The surfaces of most bacteria and archaea are covered with a proteinaceous coat, the surface or S-layer, which is formed through the self-assembly of individual protein subunits into a regularly spaced, two-dimensional array. In C. difficile, the S-layer largely consists of a major S-layer protein, SlpA, which assembles into a paracrystalline array enveloping the cell. The major protein of the C. difficile S-layer, SlpA, is post-translationally cleaved into two S-layer proteins (SLPs): the high molecular weight (HMW) and low molecular weight (LMW), herein referred to as SLPH and SLPL, respectively. These subunits then form a complex (referred to as H/L) that is incorporated in the S-layer.

The HID motif interlocks with LID in an arrangement reminiscent of a paperclip: LID α-helices α4L and α5L and HID α1H pack against a β-sheet formed by insertion of β1H from HID between LID β-strands, β18L and β21L. To identify residues essential for the interaction of the SLPL and SLPH subunits, we analyzed H/L complex formation in an enzyme-linked immunosorbent assay (ELISA) with a panel of individual point mutants. Mutations of a single amino acid within LID (F274A) or HID (Y27A) in SlpACD630 were sufficient to destabilise the H/L complex. Loss of SLPL also resulted in partial degradation of SLPH: N-terminal sequencing revealed truncation of the HID, indicating that this region is unstable in the absence of the LID/HID interaction.

>[2x]MVRVTSAKEESIDVDSSSYISAENLAKKYVFNPKEVSEAYNAIVALQNDGIESDLVQLVNGKYQVIFYPEGKRLETKS;>MADIIADADSPAKITIKANKLKDLKDYVDDLKTYNNTYSNVVLEHHHHHH[2x]>MGSSGSMVKPISGFLTALIQYPVPVVESRADIDKQIQQIIKTIHSTKSGYPGLELIVFPEYSTQGLNTKKWTTEEFLCTVPGPETDLFAEACKESKVYGVFSIMEKNPDGGEPYNTAVIIDPQGEMILKYRKLNPWVPVEPWKAGDLGLPVCDGPGGSKLAVCICHDGMFPEVAREAAYKGANVLIRISGYSTQVSEQWMLTNRSNAWQNLMYTLSVNLAGYDGVFYYFGEGQVCNFDGTTLVQGHRNPWEIVTAEVYPELADQARLGWGLENN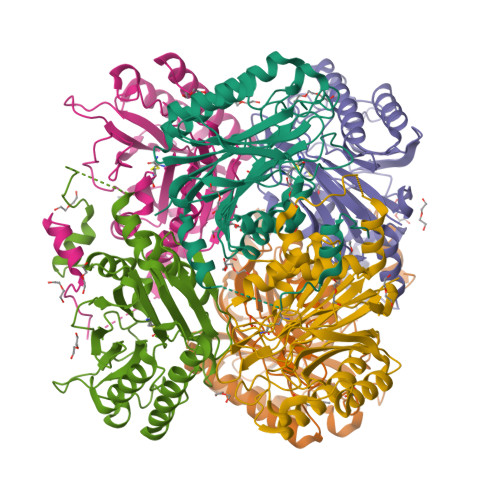IYNLGSRGYVATPGGVKENPYTFVKDLAEGKYKVPWEDEIKVKDGSIYGYPVKKTIHSWFRVDPLEHHHHHH[6x]> TAPRVVRDRDETNFHEMLGKFRFDLQGSFKENGDMLRDSLLQVGRDLFLVGWVKCRSRFATGHIQGDVHALSYMRRYLEKHVDESVSSVRFYEEN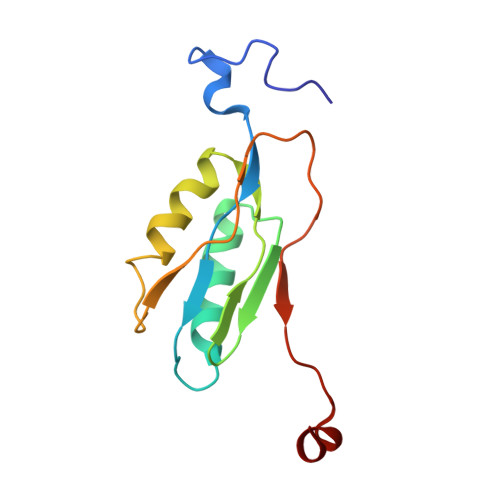FGMPLLEYERLSAVNDFRAPGKKQQH> MTENILRKSDEEIQKEITARVKALESMLIEQGILTTSMIDRMAEIYENEVGPHLGAKVVVKAWTDPEFKKRLLADGTEACKELGIGGLQGEDMMWVENTDEVHHVVVCTLCTCYPWPVLGLPPNWFKEPQYRSRVVREPRQL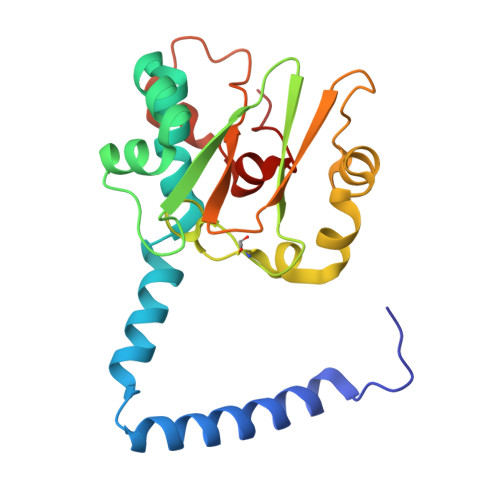LKEEFGFEVPPSKEIKVWDSSSEMRFVVLPQRPAGTDGWSEEELATLVTRESMIGVEPAKAV>[2x]GPSPNLDGTRLREEGNEAFKAGRYHEAIRYYTQAIEVDPDSEFLYTNRSFAYFNIKEFEKSAADAAKAVEINANFF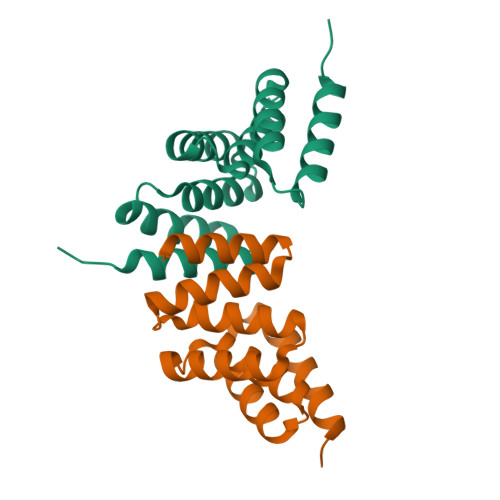KGHYRLGLAQMSLNDFGHAMESLRKAWALAPSENKEAIRVAMAKCESKMARAP> GSAASLPKRIIKETEKLVSDPVPGITAEPHDDNLRYFQVTIEGPEQSPYEDGIFELELYLPDDYPMEAPKVRFLTKIYHPNIDRLGRICLDVLKTNWSPAL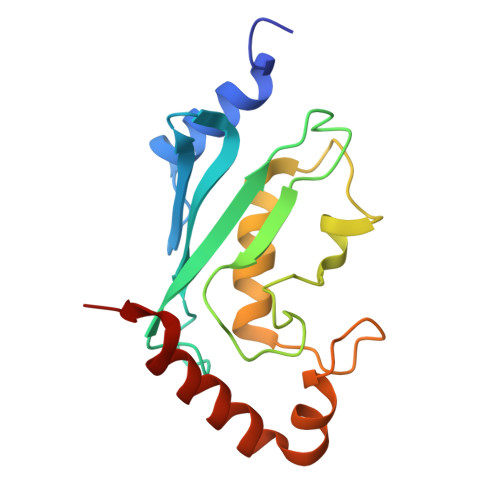QIRTVLLSIQALLASPNPNDPLANDVAEDWIKNEQGAKAKAREWTKLYAKKKPE> MMKAKVIDAVSFSYILRTVGDFLSEANFIVTKEGIRVSGIDPSRVVFLDIFLPSSYFEGFEVSQEKEIIGFKLEDVNDILKRVLKDDTLILSSNESKLTLTFDGEFTRSFELPLIQVESTQPPSVNLEFPFKAQLLTITFADIIDELSDLGEVLNIHSKENKLYFEVIGDLSTAKVELSTDNGTLLEASGADVSSSYGMEYVANTTKMRRASDSM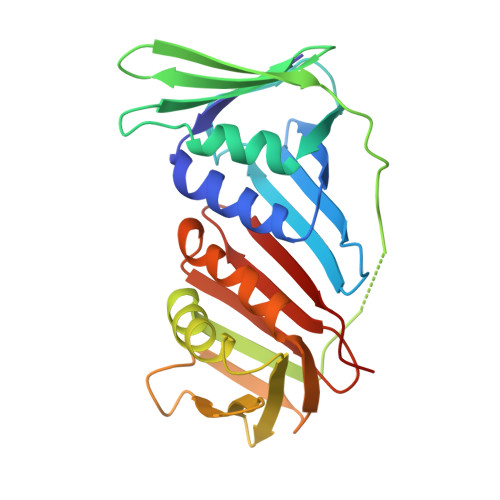ELYFGSQIPLKLRFKLPQEGYGDFYIAPRA> HSGRPVLGSSHHHHHHSSGMMLRVAVPNKGALSEPATEILAEAGYRRRTDSKDLTVIDPVNNVEFFFLRPKDIAIYVGSGELDFGIT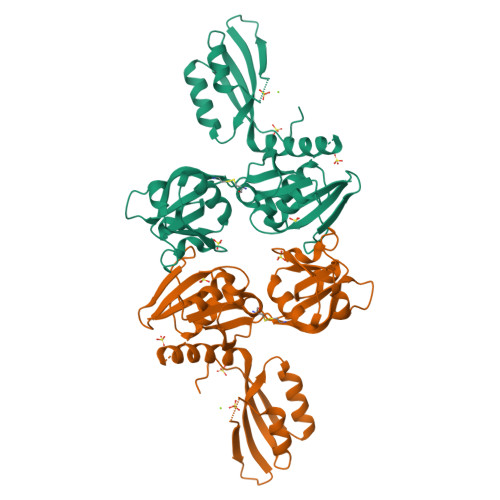GRDLVCDSGAQVRERLALGFGSSSFRYAAPAGRNWTTADLAGMRIATAYPNLVRKDLATKGIEATVIRLDGAVEISVQLGVADAIADVVGSGRTLSQHDLVAFGEPLCDSEAVLIERAGTDGQDQTEARDQLVARVQGVVFGQQYLMLDYDCPRSALKKATAITPGLESPTIAPLADPDWVAIRALVPRRDVNGIMDELAAIGAKAILASDIRFCRF>MDMLFAKTVVLAASAVGAGTAMIAGIGPGVGQGYAAGKAVESVARQPEAKGDIISTMVLGQAVAESTGIYSLVIA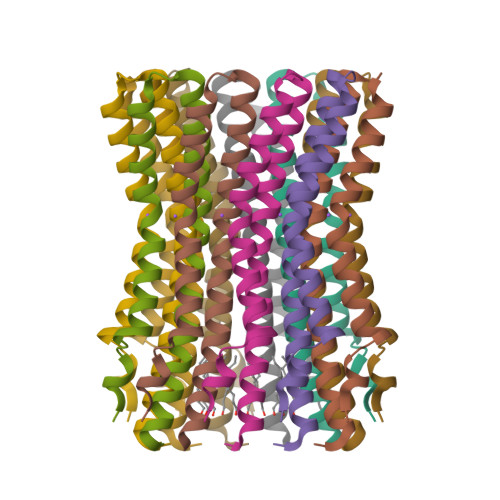LILLYANPFVGLLG[44x]> MV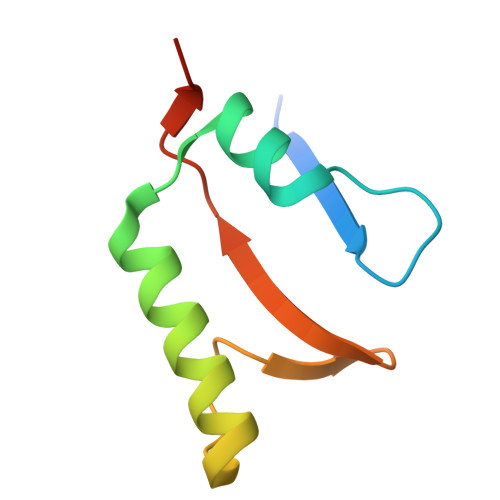RVTSAKEESIDVDSSSYISAENLAKKYVFNPKEVSEAYNAIVALQNDGIESDLVQLVNGKYQVIFYPEGKRLETKS> MNRTAPSSAALDYRSDTYRDAYSRINAIVLEGEREAHANYLTLAEMLPDHAEALKKLAAMENR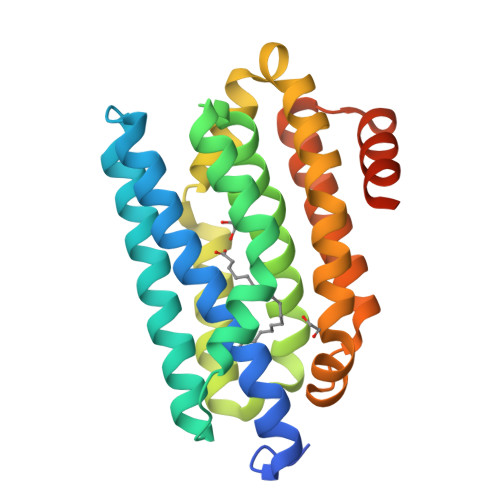HFKGFQSCARNLEVTPDDPFARAYFEQLDGNFQQAAAEGDLTTCMVIQALIIECFAIAAYNVYIPVADAFARKVTEGVVKDEYTHLNFGQQWLKERFVTVREGIERANAQNLPIVWRMLNAVEADTEVLQMDKEAIVEDFMIAYGEALGDIGFSMRDVMKMSARGLASAPRQGSHHHHHH>[2x]ENLGDLPLYHSNLFEGDIAGVSPYADKNAIVDHTLLWPGGIVYYELAPAAASIRNQILEGMKEYHEKTCIQFKERTAGVKDYIRINRYDGCWSMVG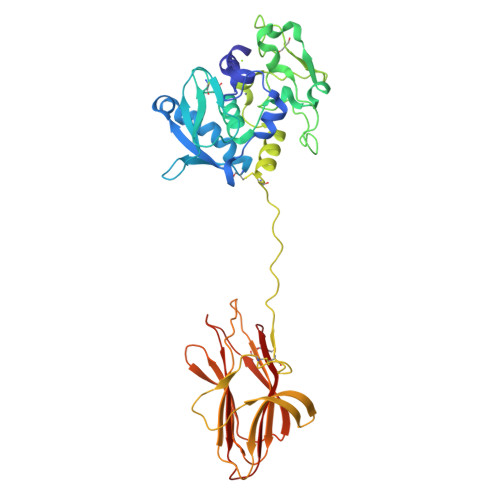RQGGMQELSLGYGCEWKGLVVHALGHAVGFWHEQNRADRDDYIEVIWDNILQSMQYNFNKMEPWENNYLNERFDYKSVMLYGETAFSKDGTSPTVRPKQPGVVIGPVWKKPGFSESDVRRVNRLYECFGEVRPPPPKIPDFICDFESNDCGLENQVGMRGEFQRKYDTLGGRTGYFMVLSVTSSGTYADSRLITPYFGAYGNQDVCMSVDVYMSGPAVRDVEISRQDSNTESIGKYTEVSNSWVTRNFNLKAGREDMRFFIFAALDPYYGDGVVAVDNLKFKRKPC>MALVDGFLELERSSGKLEWSAILQKMASDLGFSKILFGLLPKDSQDYENAFIVGNYPAAWREHYDRAGYARVDPTVSHCTQSVLPIFWEPSIYQTRKQHEFFEEASAAGLVYGLTMPLHGARGELGALSLSVEAENRAEANRFMESVLPTL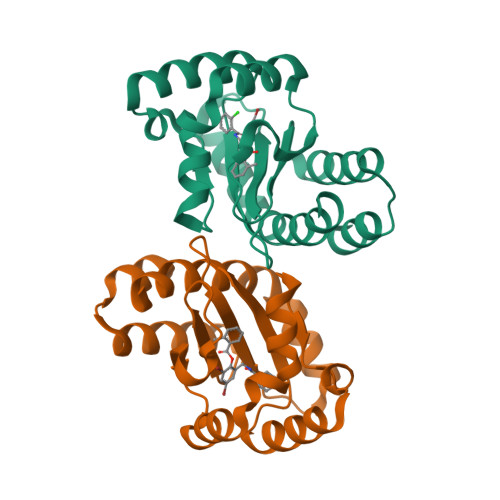WMLKDYALQSGAGLAFEHPVSK[4x]> GGACAUAUAAUCGCGUGGAUAUGGCA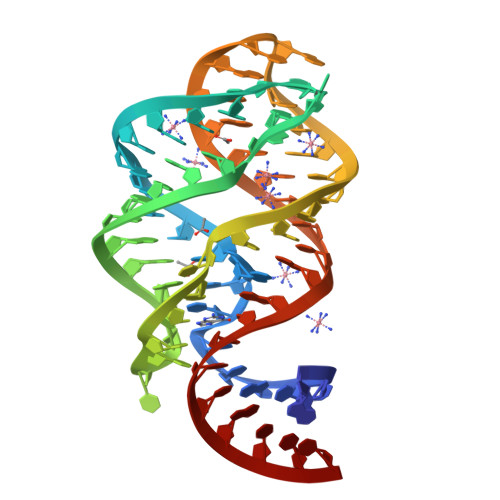CGCAAGUUUCUACCGGGCACCGUAAAUGUCCGACUAUGUCC>[2x]MADGFFKQLTLPSGQVVTVSEGRGEPASTGSYDVRLYSGANPQFPLDQFIDGKVLPRDGSIKELKLLDLNGDKQPELIVVVESAGSGSYLSADAFTLNPQ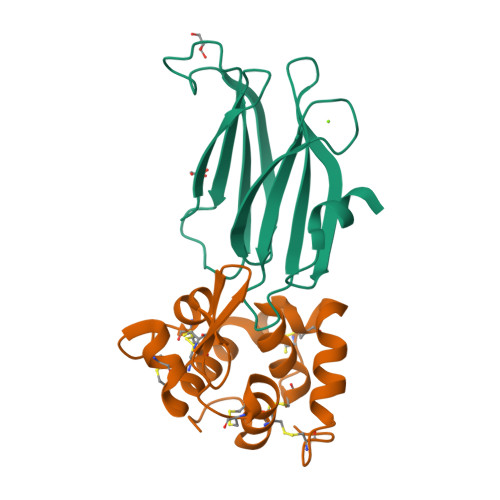EGLDSFNHVEGLAPNEDVIQALKTPRDLEHHHHHH;>[2x]FAGGIVSQRCLSCICKMESGCRNVGCKMDMGSLSCGYFQIKEAYWIDCGRPGSSWKSCAASSYCASLCVQNYMKRYAKWAGCPLRCEGFAREHNGGPRGCKKGSTIGYWNRLQKISGCHGVQ Malonyl-coenzyme A decarboxylase (MCD) is found from bacteria to humans, has important roles in regulating fatty acid metabolism and food intake, and is an attractive target for drug discovery. The MCD monomer contains an N-terminal helical domain involved in oligomerization and a C-terminal catalytic domain. Unexpectedly, the MCD catalytic domain is structurally homologous to those of the GCN5-related N-acetyltransferase superfamily, especially the curacin A polyketide synthase catalytic module, with a conserved His-Ser/Thr dyad important for catalysis. The catalytic domain of MCD contains a central eight-stranded, mostly antiparallel β sheet (β1–β8) that is surrounded by at least 11 α helices (α1–α11).

Surprisingly, CmMCD is a dimer in solution and the crystal structure reveals a completely different mode of dimerization as compared to HsMCD, RpMCD, and AvMCD. The two CmMCD monomers associate in a head-to-tail fashion such that the N-terminal helical domain of one monomer is in contact with the C-terminal catalytic domain of the other monomer, including the helical insert between strands β5 and β6. Approximately 1,100 Å2 of the surface area of each monomer is buried in this dimer. In addition, the helical hairpin insert between αC and αF is absent in CmMCD. CmMCD lacks the helical insert in the helical domain and has two additional helices between β5 and β6 in the catalytic domain, which may explain why it cannot form a similar dimer and tetramer as HsMCD or RpMCD. There is an insert of three additional helices (α5–α7) between strands β5 and β6 in HsMCD, RpMCD, and AvMCD, while CmMCD has an insert of five helices here. In the CmMCD dimer, the second monomer is located ∼20 Å away from the active site. Moreover, the loop and the following helix α4 are positioned differently in RpMCD and CmMCD, suggesting that the binding mode of CoA to these MCDs may be somewhat different unless there is a conformational change upon CoA binding in these two enzymes. After significant efforts at optimization and diffraction screening, we collected X-ray diffraction data for RpMCD, Agrobacterium vitis MCD (AvMCD), and Cupriavidus metallidurans MCD (CmMCD) at up to 2.3 Å resolution.

>[2x]STRATKRQRDQLRQCFDARLTDVAANAAAQAWQDEYEAAVEPLRQAMLGVLAEVAAVRDAAGGQPATASGLSQALSNARIRFFKRFAALHGQRGNSACGLHFLIQLRADMLRWHKRIPGLRELDEDLEALFSNWFDVGLLELQPITWDSPASLLEKLIRYEAVHEISSWTDLRNRLDSDRRCYAFFHPRIPREPLIFVEVAFVPEMAANVQALLDEAAPLEDLRRVKWAIFYSISNTQAGLRGVSFGNFLLKRVIEELQREHPKLKQFATLSPIPGFADWLRKRDGESIDRVLGVKRLARWREQHGEVPADGAAWFSALSADTEDTVIRDTAMTLAAHYLVREGGKGVPADPVARFHLGNGACVERVNWGADMSRKGRAQSCGMMVNYLYVPDALDDNLARLGDGNPRISRAVAKLLAAALEHHHHHH> GIEDLISEVAQGALTLSLPKQQDSLPDTKASGPAHSKEVPALTAVETGATNPLAPSDTVQTRHVVQRRSRSESTIESFFARGACVAIIEVDNEQPTTRAQKLFAMWRITYKDTVQLRRKLEFFTYSRFDMEFTFVVTANFTNANNGHALNQVYQIMYIPPGAPTPKSWDDYTWQTS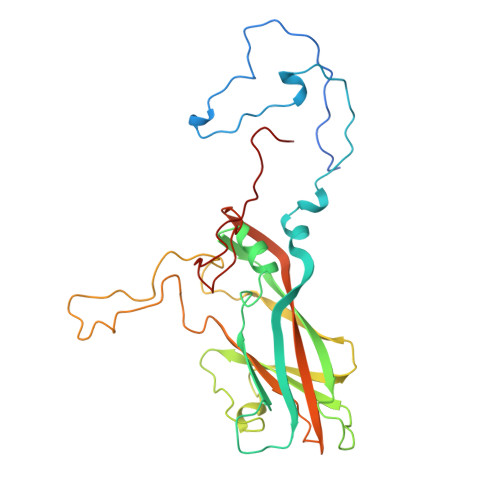SNPSIFYTYGAAPARISVPYVGLANAYSHFYDGFAKVPLKTDANDQIGDSLYSAMTVDDFGVLAVRVVNDHNPTKVTSKVRIYMKPKHVRVWCPRPPRAVPYYGPGVDYRNNLDPLSEKGLTTY>[2x]GPLGSGFEFTLMVVGESGLGKSTLINSLFLTDLYSPEYPGPSHRIKKTVQVEQSKVLIKEGGVQLLLTIVDTPGFGDAVDNSNCWQPVIDYIDSKFEDYLNAESRVNRRQMPDNRVQCCLYFIAPSGHGLKPLDIEFMKRLHEKVNIIPLIAKADTLTPEECQQFKKQIMKEIQEHKI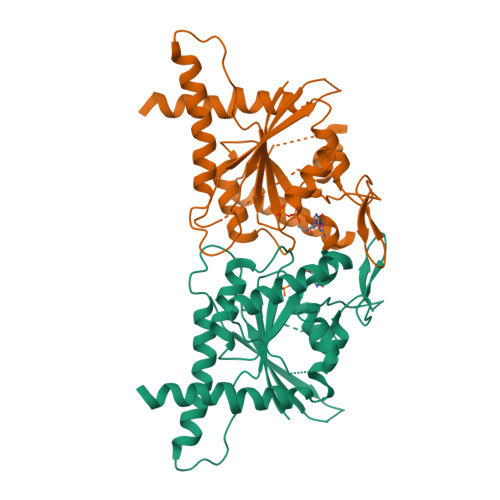KIYEFPETDDEEENKLVKKIKDRLPLAVVGSNTIIEVNGKRVRGRQYPWGVAEVENGEHCDFTILRNMLIRTHMQDLKDVTNNVHYENYRSRKLAA> AGPGWGPPRLDGFILTERLGSGTYATVYKAYAKKDTREVVAIKCVAKKSLNKASVENLLTEIEILKGIRHPHIVQLKDFQWDSDNIYLIMEFC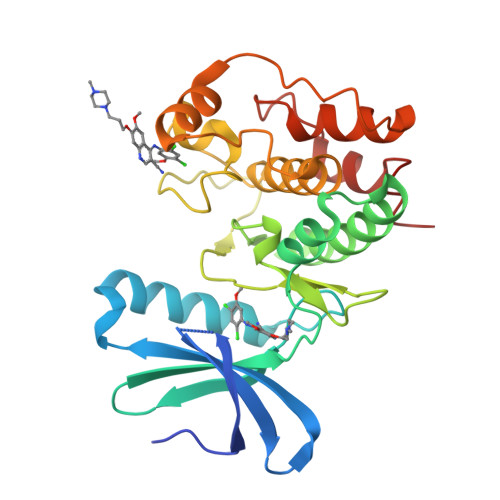AGGDLSRFIHTRRILPEKVARVFMQQLASALQFLHERNISHLDLKPQNILLSSLEKPHLKLADFGFAQHMSPWDEKHVLRGSPLYMAPEMVCQRQYDARVDLWSMGVILYEALFGQPPFASRSFSELEEKIRSNRVIELPLRPLLSRDCRDLLQRLLERDPSRRISFQDFFAHPWVDLEHMPS> MKELNDLEKKYNAHIGVYALDTKSGKEVKFNSDKRFAYASTSKAI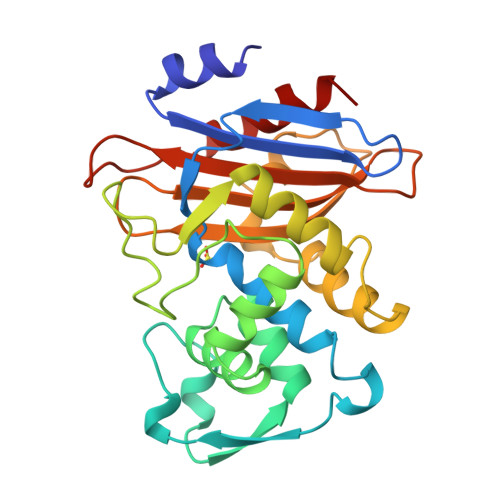NSAILLEQVPYNKLNKKVHINKDDIVAYSPILEKYVGKDITLKALIEASMTYSDNTANNKIIKEIGGIKKVKQRLKELGDKVTNPVRYQIELDYYSPKSKKDTSTPAAFGKTLNKLIANGKLSKENKKFLLDLMLNNKSGDTLIKDGVPKDYKVADKSGQAITYASRNDVAFVYPKGQSEPIVLVIFTNKDNKSDKPNDKLISETAKSVMKEF>[4x]MSYGALLFREKIPYVVEMEGDVEGMKFSVRGKGHGDANTGKIEASFICTTGELPVPWSSILTTVTYGAQCFAKYPNDIKDYPKSAMPEGYVQERTITFENDGVYKTRAEVTYEKGSVYNRVTLNGSGFKKGGNILGKKLEFNYNPHCIYVLPDVQNNGIKCYINIVHDVIGGGQIIAAHQQLNTPLGGGPVDIPHYHHIQAHTILSKDPKETRDHMNVVEVFRAIDCKTAYA

In addition to transcripts encoding an FP clearly homologous to A. victoria green fluorescent protein (avGFP), as we expected, the A. cf. australis transcriptome also contains several transcripts encoding other, much more divergent avGFP homologs. Characterization of the recombinant proteins revealed that these avGFP homologs include a green-emitting FP that appears to be the brightest FP discovered to date, 2 long-wavelength-absorbing CPs, and a reversibly photochromic FP (Figs 1Β and 2). We have identified several new Aequorea FPs with the potential to further diversify the landscape of fluorescent probes and biosensors.

We were surprised to discover a second green-emitting FP in A. cf. australis, AausFP1, that shares only 53% amino acid identity with avGFP. AausFP1 is to our knowledge the brightest FP discovered to date, with a nearly perfect quantum yield (0.97) and a peak extinction coefficient of 170,000 M−1cm−1, making it nearly 5-fold brighter than EGFP on a per-molecule basis. These already extraordinary properties are further bolstered by a low fluorescence pKa (4.4), unusually narrow excitation and emission peaks (see Fig 2; the emission peak of AausFP1 has a full width at half maximum [FWHM] of 19 nm, compared to 32 nm for EGFP), and higher photostability than mEGFP (see below). Despite low expression in its native context, wild-type AausFP1 expresses and folds very efficiently in E. coli at 37°C without any modifications. Though brightly fluorescent, AausFP1 is largely insoluble in this context, and when purified, the soluble fraction of the protein runs as a high-molecular-weight aggregate on size exclusion chromatography (Fig BB in S1 Text). X-ray crystallography revealed a uniquely stabilized chromophore environment in AausFP1 that may be responsible for its unique properties. Since AausFP1 crystallizes as a dimer, we speculate that it takes on this oligomeric state in its native context, perhaps stabilized by other interactions. It is possible that, as with other FPs such as dTomato, the dimer interface serves to stabilize the chromophore environment and may contribute to the unusually high brightness of AausFP1. AausFP1 photobleaches at similar rates to mEGFP on both widefield and confocal microscopy when instrument settings are identical, but because AausFP1 emits photons at a higher rate (due to its high quantum yield and extinction coefficient), its true photostability is somewhat higher than that of mEGFP (S1 Text and Figs Z and AA in S1 Text). AausFP1, the brightest fluorescent protein currently known, will serve as the parent of an entirely new lineage of super-bright FP variants.> MENGKRDRQDMEVNTTPRKPRVLLAASGSVAAIKFGNLCHCFTEWAEVRAVVTKSSLHFLDKLSLPQEVTLYTDEDEWSSWNKIGDPVLHIELRRWADVLVIAPLSANTLGKIAGGLCDNLLTCIIRAWDYTKPLFVAPAMNTLMWNNPFTERHLLSLDELGITLIPPIKKRLAS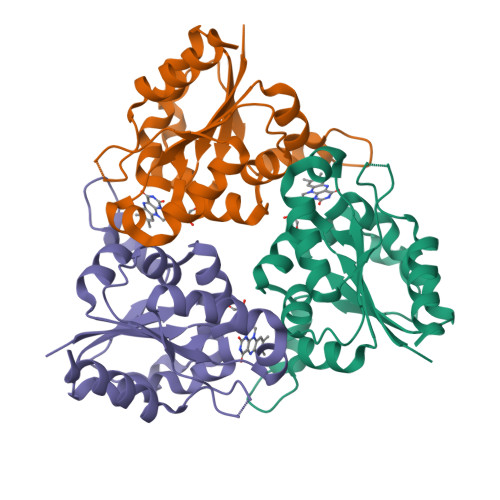GDYGNGAMAEPSLIYSTVRLFWESQAHQQTGGTS> MAEFPASLLILNGKSTDNLPLREAIMLLREEGMTIHVRVTWEKGDAARYVEEARKFGVATVIAGGGDGTINEVSTALIQCEGDDIPALGILPLGTANDFATSVGIPEALDKALKLAIAGDAIAIDMAQVNKQTCFINMATGGFGTRITTETPEKLKAALGSVSYIIHGLMRMDTLQPDRCEIRGENFHWQGDALVIGIGNGRQAGGGQQLCPNALINDGLLQLRIFTGDEILPALVSTLKSDEDNPNIIEGASSWFDIQAPHDITFNLDGEPLSGQNFHIEILPAA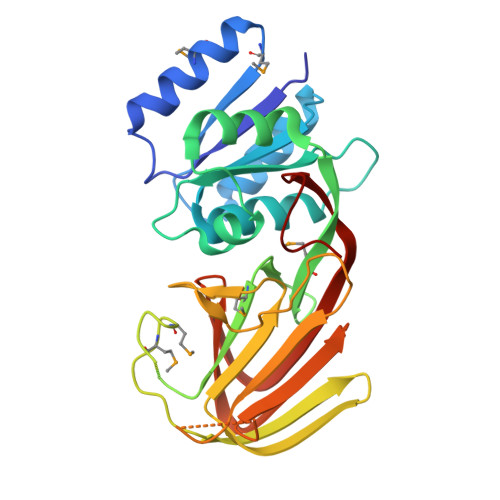LRCRLPPDCPLLR>[2x]MSLFKIRMPETVAEGTRLALRAFSLVVAVDEHGGIGDGRSIPWNVPEDMKFFRDLTTKLRGKNVKPSPAKRNAVVMGRKTWDSIPPKFRPLPGRLNVVLSSTLTTQHLLDGLPDEEKRNLHADSIVAVNGGLEQALRLLASPNYTPSIETVYCIGGGSVYAEALRPPCVHLLQAIYRTTIRASESSCSVFFRVPESGTEAAAGIEWQRETISEELTSANGNETKYYFEKLIPRNREEEQYLSLVDRIIREGNVKHDRTGVGTLSIFGAQMRFSLRNNRLPLLTTKRVFWRGVCEELLWFLRGETYAKKLSDKGVHIWDDN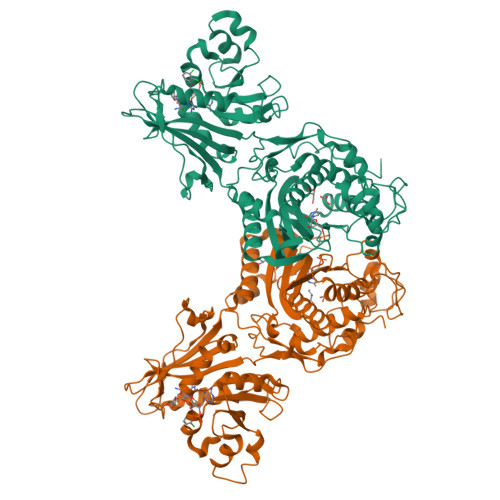GSRAFLDSRGLTEYEEMDLGPVYGFQWRHFGAAYTHHDANYDGQGVDQIKAIVETLKTNPDDRRMLFTAWNPSALPRMALPPCHLLAQFYVSNGELSCMLYQRSCDMGLGVPFNIASYALLTILIAKATGLRPGELVHTLGDAHVYSNHVEPCNEQLKRVPRAFPYLVFRREREFLEDYEEGDMEVIDYAPYPPISMKMAV> MFDGELIAKLVVELNAAMTSAQEALQFPDFEVVQKAQPTQQGTSTRPTIFFQKLFDIPRGWPATDWHLDNTARKYVEITRQHVETTFQISSLHWQNPEITHVVTASDIANYVRA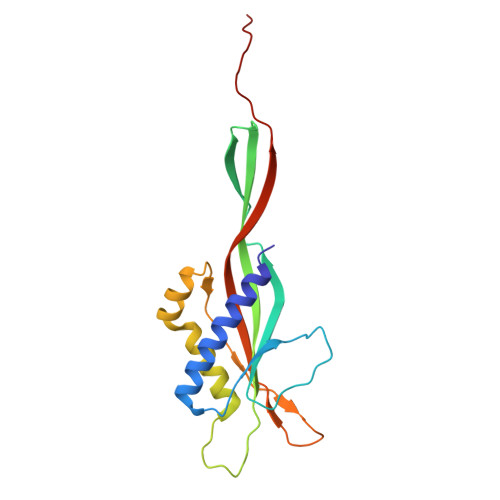YFQARSTIERVKELDFLILRVSQISNEAFENDNHQFEFHPSFDMVVTYNQYIRLYENAAYSADGVLIG> MKVISFLNPKGGSGKTTAVINIATALSRSGYNIAVVD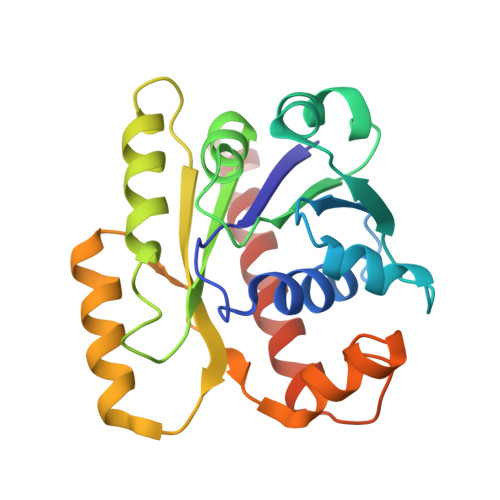TDPQMSLTNWSKAGKAAFDVFTAASEKDVYGIRKDLADYDFAIVDGAGSLSVITSAAVMVSDLVIIPVTPSPLDFSAAGSVVTVLEAQAYSRKVEARFLITRKIEMATMLNVLKESIKDTGVKAFRTAITQRQVYVKSILDGDSVFESSDGAAKGEIEILTKEIVRIFEATHHHHHH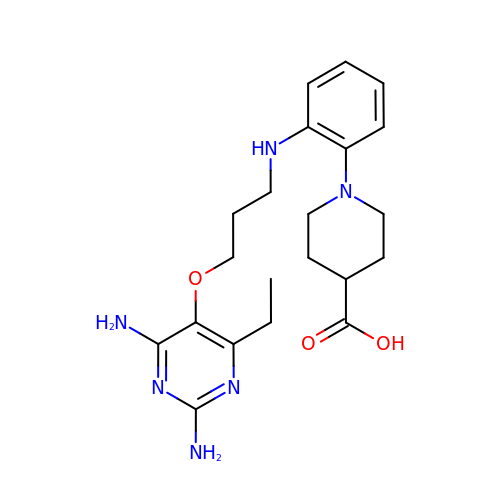1-[2-({3-[(2,4-diamino-6-ethylpyrimidin-5-yl)oxy]propyl}amino)phenyl]piperidine-4-carboxylic acid | C21 H30 N6 O3 | BQWZFCKKSJTQAP-UHFFFAOYSA-N> 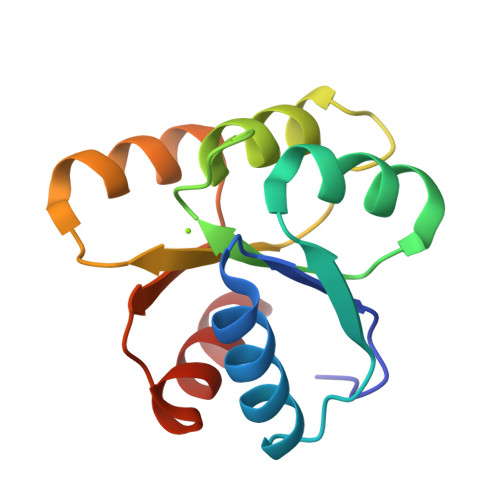ANKNMKILIVDDFSTMRRIVKNLLRDLGFNNTQEADDGLTALPMLKKGDFDFVVTDWNMPGMQGIDLLKNIRADEELKHLPVLMITAEAKREAIIEAAQAGVNGYIVKPFTAATLKEKLDKIFE>MVAKGLIRIVLDILKPHEPIIPEYAKYLSELRGVEGVNITLMEIDKETENIKVTIQGNDLDFDEITRAIESYG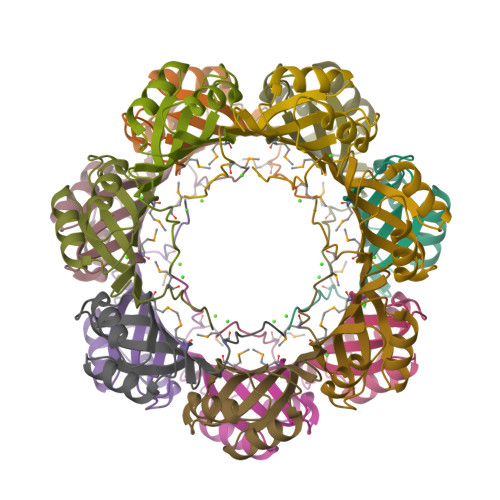GSIHSVDEVVAGRTMVEEVTTPQD[7x]>[2x]MTTAAGLSGIDLTDLDNFADGFPHHLFAIHRREAPVYWHRPTEHTPDGEGFWSVATYAETLEVLRDPVTYSSVTGGQRRFGGTVLQDLPVAGQVLNMMDDPRHTRIRRLVSSGLTPRMIRRVEDDLRRRARGLLDGVEPGAPFDFVVEIAAELPMQMICILLGVPETDRHWLFEAVEPGFDFRGSRRATMPRLNVEDAGSRLYTYALELIAGKRAEPADDMLSVVANATIDDPDAPALSDAELYLFFHLLFSAGAETTRNSIAGGLLALAENPDQLQTLRSDFELLPTAIEEIVRWTSPSPSKRRTASRAVSLGGQPIEAGQKVVVWEGSANRDPSVFDRADEFDITRKPNPHLGFGQGVHYCLGANLARLELRVLFEELLSRFGSVRVVEPAEWTRSNRHTGIRHLVVELRGG

Among these is CYP126A1, a P450 with ∼35% amino acid identity to the cholesterol-oxidizing M. tuberculosis CYP142A1 and CYP125A1. However, CYP126A1 is highly conserved across pathogenic and non-pathogenic Mycobacterium species, suggesting an important evolutionary role for the protein. In conclusion, we present the first biochemical and structural studies of the M. tuberculosis P450 CYP126A1, revealing novel substrates and inhibitors for the enzyme, defining its relatively polar active site and its ability to adapt structurally to facilitate the binding of bulky ligands. The CYP126A1 structures reveal a dynamic molecule, with the BC and FG regions clearly affected by ligand binding.

In contrast, the binding of the smaller imidazole-containing compound 7 does not lead to BC-loop reorientation, and a putative CYP126A1 dimer in complex with compound 7 in both of its active sites is observed in the asymmetric unit. The overall conformation is similar to the proposed B-B symmetric dimer, with both chains adopting a conformation resembling the imidazole-bound monomer. In addition to heme iron coordination by the compound 7 imidazole group, further contacts with CYP126A1 are limited to hydrogen bonds with Asn-96 and Ser-252 and with the ligand urea moiety, whereas the adamantyl group remains largely solvent-exposed. Although compound 7 occupies a binding pocket similar in nature to that observed for compound 1, it appears that small changes in the conformations of residues lining the compound 7 binding pocket (Gln-86 and Arg-400) lead to distinct packing interactions with the FG-helices of the opposite dimer. HTS type II compounds 7–9 produced new LS EPR spectra consistent with distal ligation of CYP126A1 heme iron by a nitrogen atom. The magnitude of change in the g-values for compounds 7–9 suggests heme coordination through the imidazole, aniline, and pyridine nitrogen atoms, respectively.(2S,4S)-4-(2,2-DIHYDROXYETHYL)-2,3,3-TRIMETHYLCYCLOPENTANONE 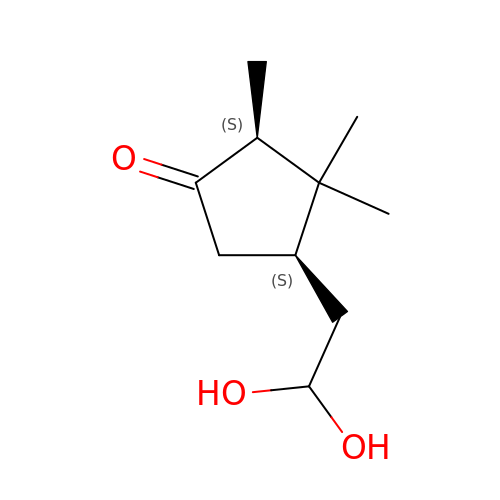| C10 H18 O3 | KAXFPJKKGITBPU-RQJHMYQMSA-N> MTLIENLNSDKTFLENNQFTDEGVKVYEFIFGENYISSGGLEATKKILSDIELNENSKVLDIGSGLGGGCMYINEKYGAHTHGIDICSNIVNMANERVSGNNKIIFEANDILTKEFPENNFDLIYSRDAILHLSLENKNKLFQKCYKWLKPTGTLLITDYCATEKENWDDEFKEYVKQRKYTLITVEEYADILTACNFKNVVSKDLSDYWNQLLEVEHKYLHENKEEFLKLFSEKKFI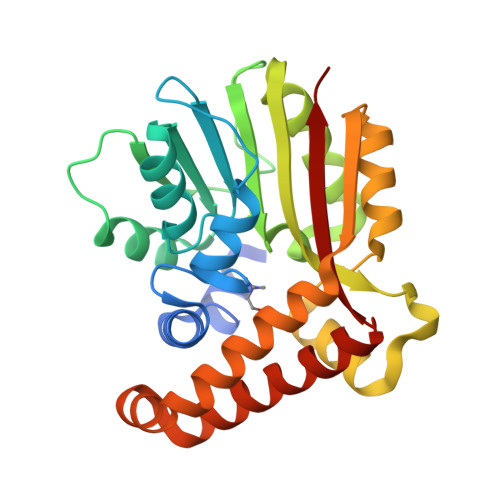SLDDGWSRKIKDSKRKMQRWGYFKATKN>[5x]AQDMVSPPPPIADEPLTVNTGIYLIECYSLDDKAETFKVNAFLSLSWKDRRLAFDPVRSGVRVKTYEPEAIWIPEIRFVNVENARDADVVDISVSPDGTVQYLERFSARVLSPLDFRRYPFDSQTLHIYLIVRSVDTRNIVLAVDLEKVGKNDDVFLTGWDIESFTAVVKPANFALEDRLESKLDYQLRISRQYFSYIPNIILPMLFILFISWTAFWSTSYEANVTLVVSTLIAHIAFNILVETNLPKTPYMTYTGAIIFMIYLFYFVAVIEVTVQHYLKVESQPARAASITRASRIAFPVVFLLANIILAFLFFGF

Pentameric ligand-gated ion channels are major mediators of fast synaptic transmission in the mammalian nervous system and serve a variety of biological roles across evolution. The extracellular domain (ECD) of each subunit contains β-strands β1–β10, with the characteristic Cys- or Pro-loop connecting β6–β7, and loops A–F enclosing a canonical ligand-binding site at the interface between principal and complementary subunits. The transmembrane domain (TMD) contains α-helices M1–M4, with M2 lining the channel pore, and an intracellular domain of varying length (2–80 residues) inserted between M3 and M4. GLIC has been thoroughly documented as a proton-gated ion channel, conducting currents in response to low extracellular pH with half-maximal activation around pH 5 (8).

To characterize the resting state of the prokaryotic pentameric channel GLIC, we first obtained single-particle cryo-EM data under resting conditions (pH 7), resulting in a map to 4.1 Å overall resolution. Local resolution was between 3.5 and 4.0 Å in the TMD, including complete backbone traces for all four transmembrane helices. Side chains in the TMD core were clearly resolved, including a constriction at the I233 hydrophobic gate (I9′, 2.9 Å Cβ-atom radius), consistent with a closed pore. Whereas some extracellular regions were similarly well resolved, local resolution in the ECD was generally lower, with some atoms that could not be definitively built in the β1–β2 loop, β8–β9 loop (loop F), and at the apical end of the ECD. At pH 7, K248 at the loop midpoint oriented down toward the M2 helix, where it could form an intrasubunit hydrogen bond with E243. In simulations of the pH-7 structure under deprotonated conditions, the K248 side chain was attracted down in each subunit towards the negatively charged E243; similar to the starting structure, these residues formed an electrostatic contact in >70% of trajectory frames. Under resting (deprotonated) conditions, negatively charged E35 attracted cations from the extracellular medium, forming a direct electrostatic contact with Na+ in >35% of simulation frames. These environmental ions were not coordinated by other protein motifs in a rigid binding site, potentially explaining poorly resolved densities in this region in neutral-pH structures. The apparent resting state (pH 7) was characterized by relatively low reconstructed resolution and flexibility in the ECD, particularly at the domain interface and peripheral surfaces, potentially conferring entropic favorability. (A) Cartoon of the GLIC resting state, corresponding to a deprotonated closed conformation, as represented by the predominant cryo-EM structure at pH 7.>MGSSHHHHHHSSGRENLYFQGMPSLTPRCIIVRAGQTEWSKSGQYTGLTDLPLTPYGEGQMLRTGESVFRNNQFLNPDNITYIFTSPRLRARQTVDLVLKPLSDEQRAKIRVVVDDDLREWEYGDYEGMLTREIIELRKSRGLDKERPWNIWRDGCENGETTQQIGLRLSRAIARIQNLHRKHQSEGRASDIMVFAHGHALRYFAAIWFGLG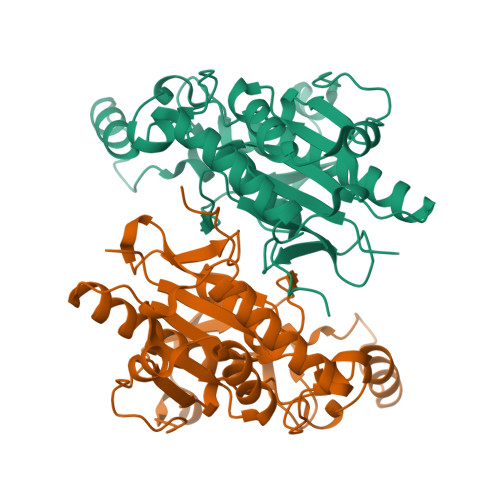VQKKCETIEEIQNVKSYDDDTVPYVKLESYRHLVDNPCFLLDAGGIGVLSYAHHNIDEPALELAGPFVSPPEEESQHGDV[2x]> SNAGKNVMVEPHRHEGVFICRGKEDALVTKNLVPGESVYGEKRVSISEGDDKIEYRAWNPFRSKLAAAILGGVDQIHIKPGAKVLYLGAASGTTVSHVSDIVGPDGLVYAVEFSHRSGRDLINLAKKRTNIIPVIEDARHPHKYRMLIAMVDVIFADVAQPDQTRIVALNAHTFLRNGGHFVISIKANCIDSTASAEAVFASEVKKMQQENMKPQEQLTLEPYERDHAVVVGVYRPPPKVKN

Fibrillarin (FBL) is an essential and evolutionarily highly conserved S-adenosyl methionine (SAM) dependent methyltransferase. It is the catalytic component of a multiprotein complex that facilitates 2′-O-methylation of ribosomal RNAs (rRNAs), a modification essential for accurate and efficient protein synthesis in eukaryotic cells. Fibrillarin consists of an N-terminal glycine–arginine-rich domain (GAR), which is believed to be important for organisation of the nucleolus, and a C-terminal domain with a Rossmann fold that is characteristic of class I S-adenosylmethionine (SAM)-dependent methyltransferases. In the present study, we determined, to our knowledge, the first crystal structures of hFBL in ligand-free state, bound to the native cofactor SAM, and in complex with two fragments that can compete with SAM for binding to the cofactor site.

In this work, we solved crystal structures of the methyltransferase domain of hFBL in apo form and in complex with the cofactor SAM. The hFBLApo and hFBLSAM structures are almost identical with an overall RMSD value of 0.2 for 229 Cα atoms, and the structures are superimposable with that of fibrillarin homolog structures from both archaeal and fungal species. Only minor changes are observed in hFBLSAM compared to hFBLApo upon SAM binding. The aromatic sidechain of F192 undergoes a significant rotation upon stacking with the adenine moiety of SAM. In addition, subtle movements in the sidechains of E191, D236, Q239, and R218 are observed upon cofactor binding. MD simulations of both hFBLApo and hFBLSAM were conducted to further examine SAM interactions with hFBL. While SAM binding showed an overall stabilising effect on hFBL structure, it appeared to destabilise the loop W137-K143, with the binding site residue R141 being the most notable.>[3x]SNAMATKL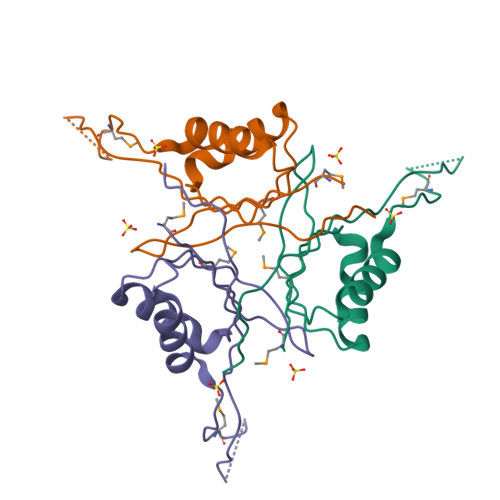VIAIVQDKDANYLSDQFIDQNVRATKLSTTGGFLQSGNTTFMIGIEEERVPEVLEIIKKASHTREEFMTPSVNMDVNMEGTTAYPIKVQVGGATVLVLPVDQFERF Cation–chloride cotransporters (CCCs) are secondary active symporters that harness the K+ and/or Na+ gradients generated by the Na+-K+-ATPase to extrude or uptake Cl− in various cell types. NKCC1 is one of the most extensively studied members of the CCC family and plays pivotal roles in trans-epithelial ion absorption and secretion, cell volume regulation, and regulation of chloride homeostasis and neuronal excitability, among others. CCCs belong to the large amino acid-polyamine-organocation (APC) superfamily of transporters. CCCs are homo- or hetero-dimers and their C-terminal domains contribute to dimer assembly.

Here, we report a cryo-EM structure of human NKCC1 captured in a partially loaded, inward-open state. We identified a human NKCC1 construct that eluted as a monodisperse peak on a size exclusion column and yielded homogenous particles suitable for 3D reconstruction by single-particle cryo-EM. This construct bears deletions in two regions (255–278 within the cytoplasmic N-terminus; 941–1000 within the cytoplasmic C-terminal domain) that are divergent among Na+-dependent CCCs, as well as two single mutations (K289N and G351R). We determined human NKCC1 transporter structure at 3.46 Å resolution that allows for de novo model building. The final map shows well-resolved densities for the transmembrane domain, large extracellular domains, and loops connecting membrane-spanning helices; however, it lacks interpretable densities for the cytosolic domains, consistent with reference free 2D class averages that show merely a cloud of fuzz densities for the cytosolic domains. NKCC1 assembles into a dimer partly via an interface formed by TM11–TM12 helices within the membrane bilayer. TM1 and TM6 helices lie at the core of the transport pathway with broken α-helical geometry roughly halfway across the lipid bilayer where two strictly conserved glycine residues may serve as flexible hinges that could facilitate the transporter to isomerize among different functional states. Ion binding sites are organized around these hinge regions with partially charged side chains, main chain atoms, and helix dipoles playing crucial roles in coordinating ions. In contrast to LeuT and many other APC transporters, NKCC1 seems to harbor multiple extracellular entryways and intracellular exits that converge at central ion binding sites, raising the possibility that K+, Na+, and Cl− ions may traverse along their own routes for translocation. We intentionally excluded K+ from our sample in order to arrest NKCC1 in a specific transport state and accordingly did not observe K+ density in our map. Using this kinetic model as a reference, our human NKCC1 structure would represent an inward-open transporter partially loaded with a Na+ and a Cl− and arrested on route before binding K+ and Cl− because K+ was excluded in sample preparation, whereas the Danio rerio NKCC1 structure represents an inward-open transporter fully loaded with K+, Na+, and Cl− ions.

>MEPRPTAPSSGAPGLAGVGETPSAAALAAARVELPGTAVPSVPEDAAPASRDGGGVRDEGPAAAGDGLGRPLGPTPSQSRFQVDLVSENAGRAAAAAAAAAAAAAAAGAGAGAKQTPADGEASGESEPAKGSEEAKGRFRVNFVDPAASSSAEDSLSDAAGVGVDGPNVSFQNGGDTVLSEGSSLHSGGGGGSGHHQHYYYDTHTNTYYLRTFGHNTMDAVPRIDHYRHTAAQLGEKLLRPSLAELHDELEKEPFEDGFANGEESTPTRDAVVTYTAESKGVVKFGWINGVLVRCMLNIWGVMLFIRLSWIVGQAGIGLSVLVIMMATVVTTITGLSTSAIATNGFVRGGRAYYLISRSLGPEFGGAIGLIFAFANAVAVAMYVVGFAETVVELLKEHSILMIDEINDIRIIGAITVVILLGISVAGMEWEAKAQIVLLVILLLAIGDFVIGTFIPLESKKPKGFFGYKSEIFNENFGPDFREEETFFSVFAIFFPAATGILAGANISGDLADPQSAIPKGTLLAILITTLVYVGIAVSVGSCVVRDATGNVNDTIVTELTNCTSAACKLNFDFSSCESSPCSYGLMNNFQVMSMVSGFTPLISAGIFSATLSSALASLVSAPKIFQALCKDNIYPAFQMFAKGYGKNNEPLRGYILTFLIALGFILIAELNVIAPIISNFFLASYALINFSVFHASLAKSPGWRPAFKYYNMWISLLGAILCCIVMFVINWWAALLTYVIVLGLYIYVTYKKPDVNWGSSTQALTYLNALQHSIRLSGVEDHVKNFRPQCLVMTGAPNSRPALLHLVHDFTKNVGLMICGHVHMGPRRQAMKEMSIDQAKYQRWLIKNKMKAFYAPVHADDLREGAQYLMQAAGLGRMKPNTLVLGFKKDWLQADMRDVDMYINLFHDAFDIQYGVVVIRLKEGLDISHLQGQEELLSSQEKSPGTKDVVVSVEYSKKSDLDTSKPLSEKPITHKVEEEDGKTATQPLLKKESKGPIVPLNVADQKLLEASTQFQKKQGKNTIDVWWLFDDGGLTLLIPYLLTTKKKWKDCKIRVFIGGKINRIDHDRRAMATLLSKFRIDFSDIMVLGDINTKPKKENIIAFEEIIEPYRLHEDDKEQDIADKMKEDEPWRITDNELELYKTKTYRQIRLNELLKEHSSTANIIVMSLPVARKGAVSSALYMAWLEALSKDLPPILLVRGNHQSVLTFYS[2x]> HMDGYYKIKHKASGKFVHPKGGSSNPPNDTNLVLHSDKHERMLFQFVDLGDGYYKIKHKASGKFVHPKGGSSNPPNDTNLVLHSDKHERMLFQFVDLGDGYYKIKHKASGKFVHPKGGSSNPPNDTNLVLHSDKHERMLFQFVDL

In 2012, a lectin designated “MytiLec” was isolated from the Mediterranean mussel Mytilus galloprovincialis, and found to bind sugar chains with α-D-galactose at the reducing end1. The polypeptide chain has three well-conserved repeats of a roughly 50-residue sequence, and adopts a β-trefoil fold. MytiLec-1 is unusual among natural β-trefoil lectins in that each sequence repeat forms a sugar-binding site, so that each polypeptide binds three identical ligands, whereas, in general, β-trefoil lectins bind only one ligand per protein subunit. Here we have adopted a similar procedure and applied it to MytiLec-1, to create a related protein with three identical subdomains, that retains sugar binding activity and the ability to bind selected cell types.

The sequence with the lowest energy score was termed “Mitsuba-1”. This 143 residue sequence includes 6 residues of the Threefoil linker, shows 61% identity with MytiLec-1, and retains the HxDxH and HPxGG motifs crucially involved in binding galactose. Analytical ultracentrifugation (AUC) shows that Mitsuba-1 is a monomer in solution, with no indication of larger species or aggregation, a result confirmed by size-exclusion column chromatography. The complex of Mitsuba-1 and NAcGal crystallised in space-group P21, and diffracted to 1.54 Å resolution. One complete monomer is found in the asymmetric unit, with no breaks in the the 2mFo-DFc electron density map of the chain, and there are no Ramachandran outliers. The structure is well ordered with each subdomain forming a β-sheet of four strands. Overlaying 143 Cα atoms of Mitsuba-1 and MytiLec-1 gives an RMSD value of 0.86 Å, showing the structures are highly related. The three-fold symmetry prevents internal residues of Mitsuba-1 from approaching the symmetry axis too closely, and a central cavity is found in the structure with a volume close to 100 Å3 according to KVFinder25. Three GalNAc ligands are found at shallow binding sites related by the three-fold symmetry of the protein. The contacts between Mitsuba-1 with GalNAc include five hydrogen bonds, including hydrogen bonds with two histidines and two aspartate residues. The HxDxH motif found at each binding site of MytiLec-1 is preserved, so that His 33, His 81 and His 129 of Mitsuba-1 form van der Waals contacts with the ligands but make no hydrogen bond with them.>[2x]XKKLLKC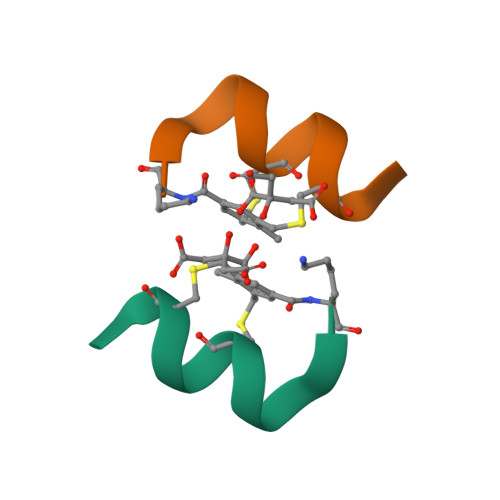LKCLLX>VSRIVVHTRWASNVDFDRDSSVIMAPPTENNIHLFKQLLNTETLSVRGANPLMFRANVLHMLLEFVLDNLYLNRHTGFSQDHTPFTEGANLRSLPGPDAEKWYSIMYPTRMGTPNVSKICNFVASCVRNRVGRFDRAQMMNGAMSEWVDVFETSDALTVSIRGRWMARLARMNINPTEIEWALTECAQGYVTVTSPYAPSVNRLMPYRISNAERQISQIIRIMNIGNNATVIQPVLQDISVLLQRISPLQIDPTIISNTMSTVSESTTQTLSPASSILGKLRPSNSDFSSFRVALAGWLYNGVVTTVIDDSSYPKDGGSVTSLENLWDFFILALALPMTTDPCAPVKAFMTLANMMVGFETIPMDNQIYTQSRRASAFSTPHTWPRCFMNIQLISPIDAPILRQWAEIIHRYWPNPSQIRYGAPNVFGSANLFTPPEVLLLPIDHQPANVTTPTLDFTNELTNWRARVCELMKNLVDNQRYQPGWTQSLVSSMRGTLDKLKLIKSMTPMYLQQLAPVELAVIAPMLPFPPFQVPYVRLDRDRVPTMVGVTRQSRDAITQPALSLSTTNTTVGVPLALDARAITVALLSGKYPPDLVTNVWYADAIYPMYADTEVFSNLQRDMITCEAVQTLVTLVAQISDTQYPVDRYLDWIPSLRASAATAATFAEWVNTSLKTAFDLSDMLLEPLLSGDPRMTQLAIQYQQYNGRTFDVIPEMPGSVIADCVQLTAEVFNHEYNLFGIARGDIIIGRVQ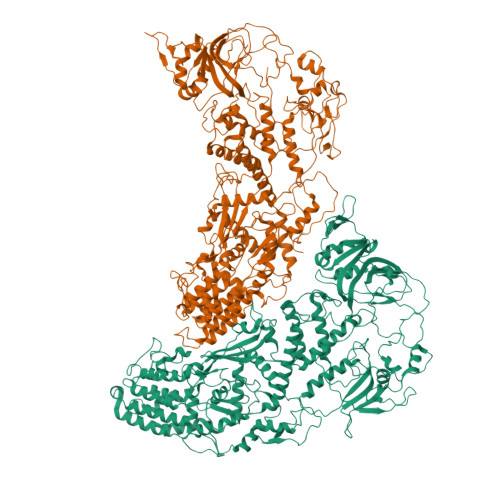STHLWSPLAPPPDLVFDRDTPGVHIFGRDCRISFGMNGAAPMIRDETGMMVPFEGNWIFPLALWQMNTRYFNQQFDAWIKTGELRIRIEMGAYPYMLHYYDPRQYANAWNLASAWLEEITPTSIPSVPFMVPISSDHDISSAPAVQYIISTEYNDRSLFCTNSSSPQTIAGPDKHIPVERYNILTNPDAPPTQIQLPEVIDLYNVVTRYAYETPPITAVVMGVP[2x]>[2x]GHMPNIPPPFTAPYAPDDAEIAARLLPASHLSPPQEARIHRTATRLIEAIRKRDDRLGGVEDMLREFALSTKEGLALMVLAEALLRVPDARTADQFIEDKLGEGDFIHHETKSTAFLVNASAWALGLSARVIQPGETPDGTIGRLVKRLGAPAVRTATRQAMRLMGNHFVLGETIEQALERGKPRSGQKTRYSFDMLGEGARTAADARRYFDAYASAIETIGKAAGNHALPDRPGISVKLSALHPRFEAISRARVMVELVPQLLDLAQRAKAHDLNFTVDAEEADRLELSLDVIAATLADPSLKGWDGFGLAIQAYQKRASAVIDYVDALARAHDRKLMVRLVKGAYWDTEIKRAQERGLDGYPVFTRKAMTDLNYVACASKLLALRPRIFPQFATHNALTVATVLEMAEGSSGFEFQRLHGMGEALYEQLAKDHADIAYRTYAPVGSHRDLLAYLVRRLLENGANSSFVAQAADYRVPVPALLQRPADAIVRPQAA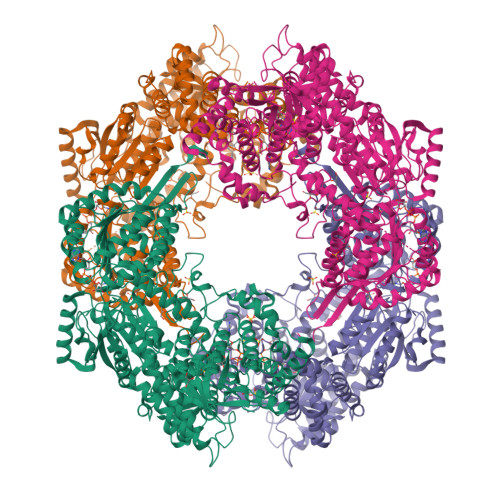AHPRIPLPCDLFAPERRNSRGVEFGARTALDQLLTDVKAETGDLKPIADATPDQAHAAVAAARAGFAGWSRTPAGIRAAALEQAAHLLESRSAHFIALLQREGGKTLDDALSELREAADFCRYYAAQGRKLFGSETAMPGPTGESNALTMRGRGVFVAISPWNFPLAIFLGQVTAALMAGNSVVAKPAEQTPRIAREAVALLHEAGIPKSALYLVTGDGRIGAALTAHPDIAGVVFTGSTEVARSINRALAAKDGPIVPLIAETGGINAMIADATALPEQVADDVVTSAFRSAGQRCSALRLLFVQEDVADRMIEMVAGAARELKIGDPSDVATHVGPVIDVEAKQRLDAHIARMKTEARLHFAGPAPEGCFVAPHIFELTEAGQLTEEVFGPILHVVRYRPENLERVLRAIERTGYGLTLGVHSRIDDSIEAIIDRVQVGNIYVNRNMIGAVVGVQPFGGNGLSGTGPKAGGPHYLARFATEQTVTINTAAAGGNAALLAGEE> MASKKENLKSLFSNTRTRVIIIFTAALLIIAVVIGFFKIRGATTGSIAAAEVSTVPGGIQSIPGVLDPTAQYAKLQEEQNITQAQVAEKTGGSAIPTIIRTQALGEGVGVIGSQSGVGFAALAQEELGGPQRSLWIQELQDGSCSKSVITKVVNQGAQLTDLKAACSCVQLKDSGYGLQELEQVCECKELKSAGYNARQLKEAGYSAGRLRNCGFDACELRNAGFTAQEMKDGGFSDGELKGAGFSDAEIAKASGLPDGITADDVRKAGCGAAALAKLRQAGVSASAIRKISGCTAEQLKAAGYTAKELKDAGFSAADLRRAGFSAAELKDAGFTARDLLNAGFTPADLAKAGFSDAQIKAAQAELPPGITPQDVKNAGCDVEALKKEREAGVSAALIRQYAGCSAQALKAAGFTDADLANAGFTPAQISAATP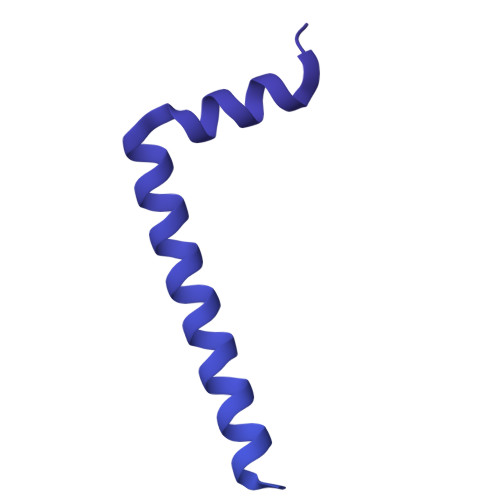LSDAEIKAAGCDPDKLKKLFSAGVSAKRIKELNGCSAEALKAAGYDAQSLLAAGFTPQELLAAGFTPKQLEDAGLNPVSIIADGRVADCSVESLKKARAAGVSALTIKQTLGCSAAALKAAGYTAKELKDAGFTAAELKAAGFSAKELKDAGFTAKELRDAGFSAQELKDVGFSAKDLKDAGFSAAELKAAGFTAAQLKAAGFSAKDLKDAGFSAAELKAAGFSAKELKDAGFSASDLKNAGFSAKELKDAGFSASDLKSAGFSASELKNAGYSADELKKAGYTSAELRNAGFSPQESAVAGLQGPDLQQLDSSITGIPSIPGATPRPTTSDAASSAEQLQAILQKQNEQLAEQKYQQEIQQRTSDMLTAATQLVQDWKQVETQVYTEGTEETKTSGGESAVPGTGTGTGSNNQPVDQGAVSAQNQAIIKTGDIMFAVLDTSVNSDEPGPILATIVTGKLKGSKLIGSFNLPSNADKMVITFNTMSIPGAEKTISISAYAIDPNTARTALASRTNHHYLMRYGSLFASSFLQGFGNAFQSANTTITIGGTGGGNNITVANGVGRSTLENAVIGLATVGKAWSQQAQQLFNTPTTVEVYSGTGLGILFTQDVTTI>[12x]MPSGYGVLLATHDDDTVDVFTSGRKMRLTCSPNIDAASLKKGQTVRLNEALTVVEAGTFEAVGEIS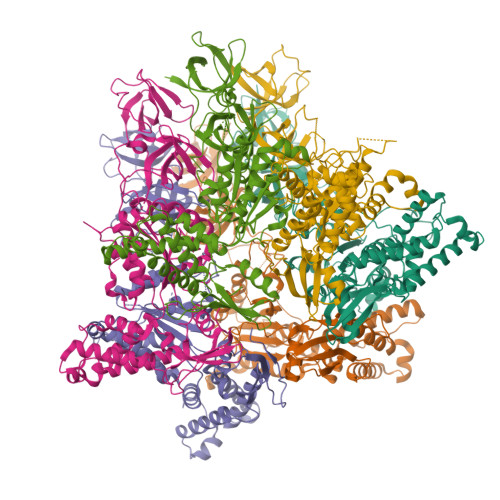TLREILADGHRALVVGHADEERVVWLADPLIAEDLPDGLPEALNDDTRPRKLRPGDSLLVDTKAGYAFERIPKAEVEDLVLEEVPDVSYADIGGLSRQIEQIRDAVELPFLHKELYREYSLRPPKGVLLYGPPGCGKTLIAKAVANSLAKKMAEVRGDDAHEAKSYFLNIKGPELLNKFVGETERHIRLIFQRAREKASEGTPVIVFFDEMDSIFRTRGTGVSSDVETTVVPQLLSEIDGVEGLENVIVIGASNREDMIDPAILRPGRLDVKIKIERPDAEAAQDIYSKYLTEFLPVHADDLAEFDGDRSACIKAMIEKVVDRMYAEIDDNRFLEVTYANGDKEVMYFKDFNSGAMIQNVVDRAKKNAIKSVLETGQPGLRIQHLLDSIVDEFAENEDLPNTTNPDDWARISGKKGERIVYIRTLVTGKSSSASRAIDTESNLGQYL> GLMDEGLPPEEVERIRAFLQERIRGRALE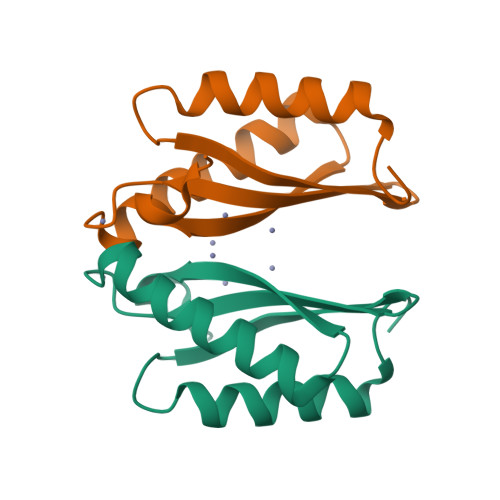VHDLKTRRAGPRSFLEFHLVVRGDTPVEEAHRLCDELERALAQAFPGLQATIHVEPEGERKRTNP>FTLIELAIVIVIIGILVAIAVPRFVDLTDQANQANVDATAAAVRSAYAIATVQAKGIPTCDQVFANPEGGSTSGSTWTSSDNSTTVSCNASADTFTISRGGKTRTLNLTVN[16x]

Type IV pili (T4P) are flexible extracellular protein filaments found on many bacteria. They form multifunctional fibres involved in twitching motility, adhesion, immune evasion, bacteriophage infection, virulence and colony formation. Pilins have a conserved N-terminal α-helix, with a 4–5 stranded antiparallel β-sheet at the C-terminus. The α-helix forms the core of the filament, while the globular β-sheet head domain is solvent exposed and subject to post-translational modification.

Proteomics and knock-out mutants reveal that the narrow pilus consists of a previously unknown pilin, which we name PilA5. In contrast, the narrow pilus has a zigzag-like appearance in projection, owing to a 15 Å wide groove that winds through the filament. The diameter at any position along the long axis of the filament is therefore only 45 Å. The glycosylation loop in PilA5 spans amino acids 54–71, with amino acids 62 to 65 forming a one-turn helix. The C-terminal β-sheet is composed of five strands, one more than observed in PilA4. A disulphide bond is formed between Cys60 in the glycosylation loop and Cys88 in the third β-strand. In contrast, PilA5 has a total of 2 negative charges per subunit which leads to a patch of negative charge winding around the filament. In contrast, PilA5 contains a single intermolecular salt bridge—between Glu68 (subunit A) and Arg23 (subunit D). Supported by our curvature analysis, narrow pili comprised of PilA5 appear to be more flexible than those comprised of PilA4. We determine two functions for PilA5: it forms the main structure of the narrow T4P and is a requirement for cell motility.>CCGTAATGCC[4x];>[4x]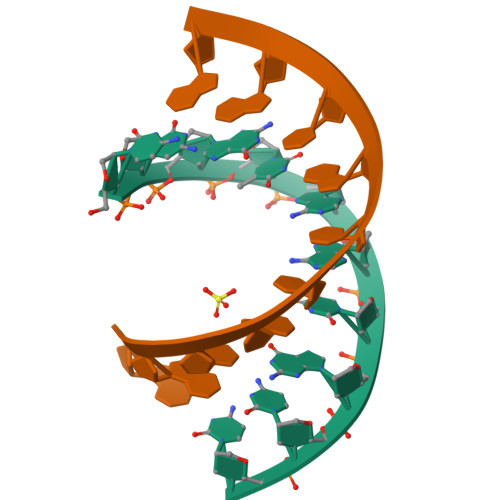GGCAUUACGG>MHHHHHHGTQQEALGMVETKGLTAAIEAADAMVASANVMLVGYEKIGHGLVTVIVRGDVGAVKAATDAGAAAARNVGEVKAVHVIPRPHTDV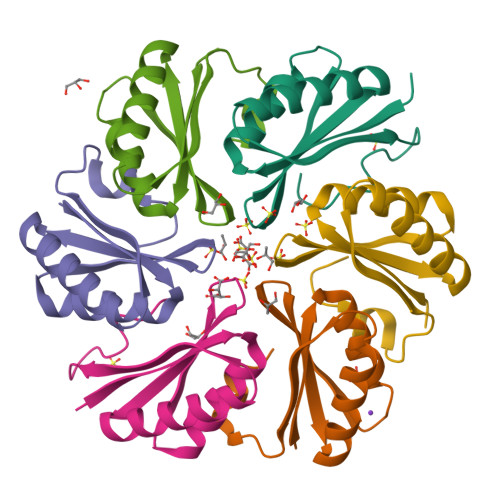EKILPKGISQ[9x]> MANKNYQMSTGVTAVVQKVVEACQDESKRLDLIEIARSYPPNQLRNMQRTFQAITGTFLDAFLKKHLSKDFESLVLMLYKPRAQLLCELIRGATKGAGTDEKCLVDVLLTIETHEVREIRQLYYQLYNDSLGDVVRKDCGDKYMWAKLINAVATGDRIPRDTHELEEDLVLVRKAIETKGVKKDEVSTWIRIFATYTRAD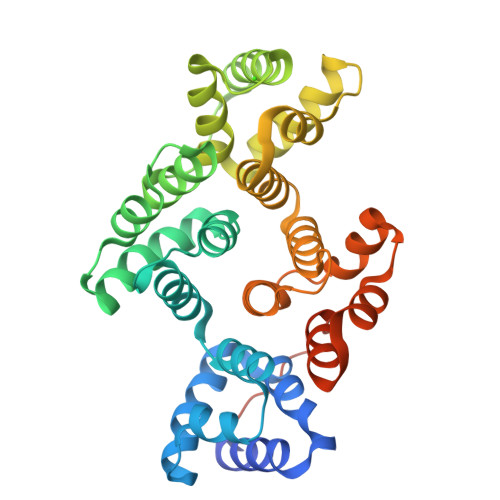FRQLHKMYSAKYNGDSLRAGVEDEFQGLDEYAFKLAHDFLYDPCCAAAFSMNVAFAGSGSDSNRLNRITAMHFRECKGCKYYYKKVYGQAFDERCATELKGVYGDAIKLLWEPVTVPLLSMDDYQGSEQHRPMTLEL O-[(1R,2R,3R)-5-{[(S)-{[(2R,3R,4R,5R)-2-(2-amino-6-oxo-3,6-dihydro-9H-purin-9-yl)-4-hydroxy-5-(hydroxymethyl)tetrahydrofuran-3-yl]oxy}(sulfanyl)phosphoryl]oxy}-1-(6-amino-9H-purin-9-yl)-1,2-dihydroxypentan-3-yl] dihydrogen (R)-phosphorothioate | C20 H28 N10 O12 P2 S2 | 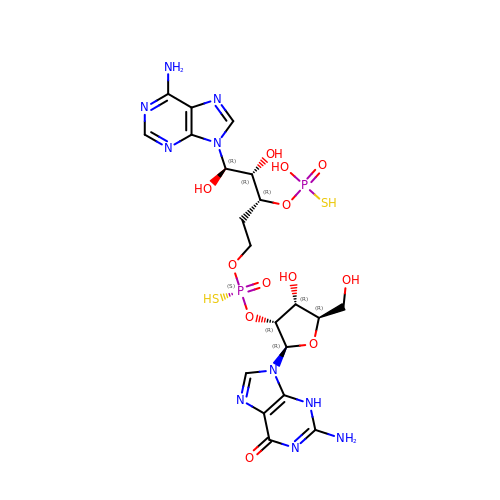WDMUGQSSXDUMIY-MHPWAGLLSA-N> MATVEPETTPTPNPPTTEEEKTESNQEVANPEHYIKHPLQNRWALWFFKNDKSKTWQANLRLISKFDTVEDFWALYNHIQLSSNLMPGCDYSLFKDGIEPMWEDEKNKRGGRWLITLNKQQRRSDLDRFWLETLLCLIGESFDDYSDDVCGAVVNVRAKGDKIAIWTTECENREAVTHIGRVYKERLGLPPKIVIGYQSHADTATKSGSTTKNRFVV;> MATVEPETTPTPNPPTTEEEKTESNQEVANPEHYIKHPLQNRWALWFFKKDKSKTWQANLRLISKFDTVEDFWALYNHIQLSSNLMPGCDYSLFKDGIEPMWEDEKNKRGGRWLITLNKQQRRSDLDRFWLETLLCLIGESFDDYSDDVCGAVVNVRAKGDKIAIWTTE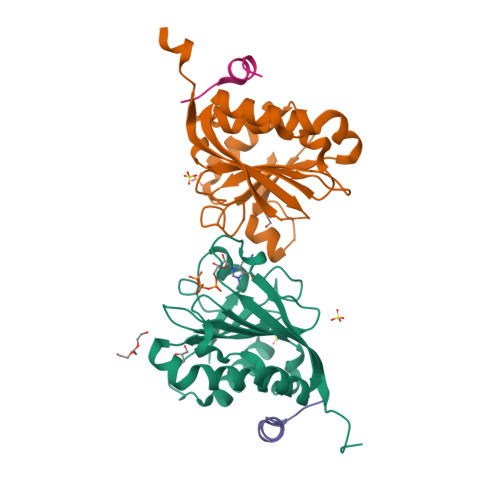CENREAVTHIGRVYKERLGLPPKIVIGYQSHADTATKSGSTTKNRFVV;>KKRYDREFLLGFQF[2x]>MEGISIYTSDNYTEEMGSGDYDSMKEPCFREENANFNKIFLPTIYSIIFLTGIVGNGLVILVMGYQKKLRSMTDKYRLHLSVADLLFVITLPFWAVDAVANWYFGNFLCKAVHVIYTVNLYSSVLILAFISLDRYLAIVHATNSQRPRKLLAEKVVYVGVWIPALLLTIPDFIFANVSEADDRYICDRFYPNDLWVVVFQFQHIMVGLILPGIVILSCYCIIISKLSHSKGHQKRKALKTTVILILAFFACWLPYYIGISIDSFILLEIIKQGCEFENTVHKWISITEALA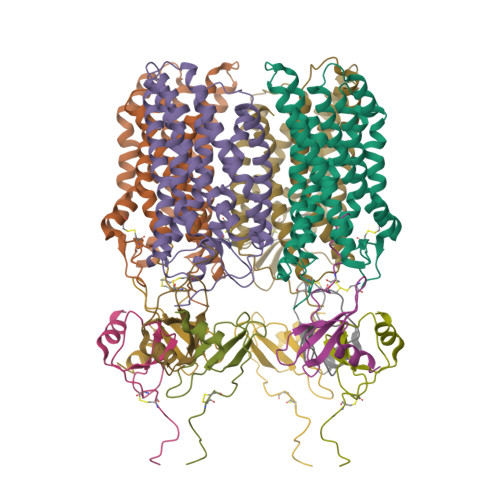FFHCCLNPILYAFLGAKFKTSAQHALTSVSRGSSLKILSKGKRGGHSSVSTESESSSFHSSDYKDDDDK[4x];>[8x]KPVSLSYRCPCRFFESHVARANVKHLKILNTPNCALQIVARLKNNNRQVCIDPKLKWIQEYLEKALNKRFKMHHHHHHHH> GSHMSSAFGAETVLEVRHWTDAYFSFTTTRDAGFRFENGQFVMIGLETETRPLLRAYSIASANWEEHLEFFSIKVPDGPLTSRLQHIQPGDKVLVGKKPTGTLLISDLHPGRNLYLLGTGTGLAPWLSIIKDPETYERFDKVILTQGVRFVQDLAYRDYFERELPQHEFLGDLLREKLLYYPAVTRETFANQGRLTELMADGRMQQTLGLPTLDPANDRFMICGSPQMLADLRSLLDSRGFQTSPRIGTPGHYVFERAFVEK

Ferredoxin-NADP(H) reductases (FNRs, EC 1.18.1.2) constitute a family of hydrophilic FAD-containing monomeric enzymes that deliver NADPH or low potential one-electron donors to redox-based metabolisms in plastids, mitochondria, and bacteria. Structures of bacterial FPRs, as well as those of plastidic FNRs, are folded in two distinct domains: the C-terminus with a binding site for NADP(H) and the N-terminus binding the cofactor FAD. The genome of X. axonopodis pv. citri contains the fpr gene that encodes the FPR (XacFPR). Despite the fact that neither the role of XacFPR nor its potential substrate has been elucidated, its involvement in the oxidative stress response of X. axonopodis pv. citri via interaction with ferredoxin XAC1762 has been proposed.

We here report the crystal structure of XacFPR at a resolution of 1.5 Å. The overall structure of XacFPR strongly resembles those of bacterial FPRs from subclass I. It is organised in the two typical domains present in the ferredoxin-NADP(H) reductase family. The N-terminus (residues 4–98) folds into a six-stranded antiparallel β-barrel (β1–β6) capped by helix α1. FAD binds to this domain, near the N-terminal end of α1 and the carboxy ends of the strands β4 and β5. The C-terminus (residues 99–259) adopts a classical nucleotide binding fold with a five-stranded parallel β-sheet surrounded by nine α-helices. Finally, a chloride ion coming from the crystallization mother liquor is located between helices α8 and α10, at the C-domain, stabilised by the OG1 atom of Thr193 and two water molecules. Subclass IA FPRs, to which XacFPR belongs, are characterised by the short C-terminal sequence VEK. The C-terminal glutamic residue side chain (Glu258, numbering as in XacFPR) establishes an interaction with the O2′ of the FAD ribityl in the XacFPR and Pseudomonas aeruginosa FPR (PaFPR) structures, but not in that of A. vinelandii FPR (AvFPR). Finally, in XacFPR, the exposure of FAD to the solvent is limited by interaction of the phosphoadenosine phosphate moiety of the cofactor with the side chain of Lys259, probably introducing structural restrictions to the enzyme catalytic turnover. Here we describe the first crystal structure of XacFPR. This structure shows structural features that correspond to a protein from bacterial subclass IA but with detectable differences in the mobility of specific loops when compared with other known bacterial FPRs.> MTGREILEKLERREFTREVLKEALS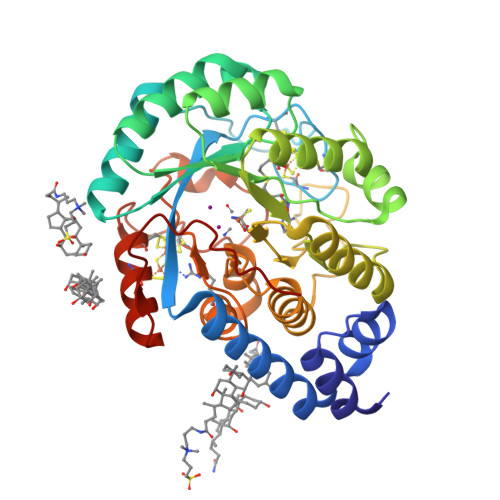INDRGFNEALFKLADEIRRKYVGDEVHIRAIIEFSNVCRKNCLYCGLRRDNKNLKRYRMTPEEIVERARLAVQFGAKTIVLQSGEDPYYMPDVISDIVKEIKKMGVAVTLSLGEWPREYYEKWKEAGADRYLLRHETANPVLHRKLRPDTSFENRLNCLLTLKELGYETGAGSMVGLPGQTIDDLVDDLLFLKEHDFDMVGIGPFIPHPDTPLANEKKGDFTLTLKMVALTRILLPDSNIPATTAMGTIVPGGREITLRCGANVIMPNWTPSPYRQLYQLYPGKICVFEKDTACIPCVMKMIELLGRKPGRDWGGRKRVFETV>AGFANIQGRADLSDVHLPDQVIKDVLQTAPEASVLLNRARKVRMSSKKTKQPVLASLPDAYWVDGDTGLKQTTKNIWSNVFMTAEELAVIVPIPDALIADSDLPLWDEVKPLLVEAIGKKVDDAGIFGNDKPASWPAALIPGAIAAGNSVTLGTGDDIGVDVATLGEQLALDGFSINGFISRPGLHWSLVGLRNAQGQPIYTPPLSTGLNGAPPTPALYGFPLNEVTSGVWDADEAILLGADWSKVVIGIRQDITFDLFS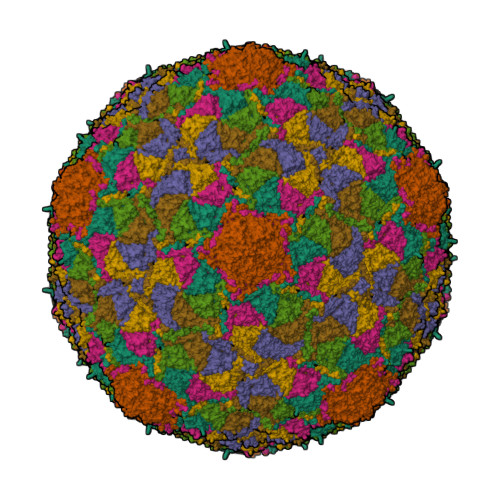EGVISDSDGKVVLNLMQQDSKALRVVFRVGFQVANPMTRLNPNEATRYPAGVIIPAGGGSGEGEGESE[7x]3-{[(1Z)-1-carboxyprop-1-en-1-yl]oxy}-2-hydroxybenzoic 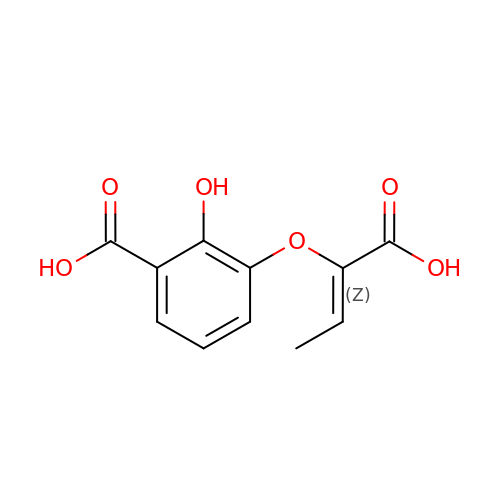acid | C11 H10 O6 | MPHSNGOSXHODDD-UQCOIBPSSA-N>MAAPVVAPPGVVVSRANKRSGAGPGGSGGGGARGAEEEPPPPLQAVLVADSFDRRFFPISKDQPRVLLPLANVALIDYTLEFLTATGVQETFVFCCWKAAQIKEHLLKSKWCRPTSLNVVRIITSELYRSLGDVLRDVDAKALVRSDFLLVYGDVISNINITRALEEHRLRRKLEKNVSVMTMIFKESSPSHPTRCHEDNVVVAVDSTTNRVLHFQKTQGLRRFAFPLSLFQGSSDGVEVRYDLLDCHISICSPQVAQLFTDNFDYQTRDDFVRGLLVNEEILGNQIHMHVTAKEYGARVSNLHMYSAVCADVIRRWVYPLTPEANFTDSTTQSCTHSRHNIYRGPEVSLGHGSILEENVLLGSGTVIGSNCFITNSVIGPGCHIGDNVVLDQTYLWQGVRVAAGAQIHQSLLCDNAEVKERVTLKPRSVLTSQVVVGPNITLPEGSVISLHPPDAEEDEDDGEFSDDSGADQEKDKVKMKGYNPAEVGAAGKGYLWKAAGMNMEEEEELQQNLWGLKINMEEESESESEQSMDSEEPDSRGGSPQMDDIKVFQNEVLGTLQKGKEENISCDNLVLEINSLKYAYNISLKEVMQVLSHVVLEFPLQQMDSPLDSSRYCALLLPLLKAWSPVFRNYIKRAADHLEALAAIEDFFLEHEALGISMAKVLMAFYQLEILAGETILSWFSQRDTTDKGQQLRKNQQLQRFIQWLKEAEEESSEDD[2x];>MHHHHHHGGGSENLYFQSPGSAAKGSELSERIESFVETLKRGGGPRSSEEMARETLGLLRQIITDHRWSNAGELMELIRREGRRMTAAQPSETTVGNMVRRVLKIIREEYGRLHGRSDESDQQESLHKLLTSGGLNEDFSFHYAQLQSNIIEAINELLVELEGTMENIAAQALEHIHSNEVIMTIGFSRTVEAFLKEAARKRKFHVIVAECAPFCQGHEMAVNLSKAGIETTVMTDAAIFAVMSRVNKVIIGTKTILANGALRAVTGTHTLALAAKHHSTPLIVCAPMFKLSPQFPNEEDSFHKFVAPEEVLPFTEGDILEKVSVHCPVFDYVPPELITLFISNIGGNAPSYIYRLMSELYHPDDHVL[2x];>[2x]MAAVAVAVREDSGSGMKAELPPGPGAVGREMTKEEKLQLRKEKKQQKKKRKEEKGAEPETGSAVSAAQCQVGPTRELPESGIQLGTPREKVPAGRSKAELRAERRAKQEAERALKQARKGEQGGPPPKASPSTAGETPSGVKRLPEYPQVDDLLLRRLVKKPERQQVPTRKDYGSKVSLFSHLPQYSRQNSLTQFMSIPSSVIHPAMVRLGLQYSQGLVSGSNARCIALLRALQQVIQDYTTPPNEELSRDLVNKLKPYMSFLTQCRPLSASMHNAIKFLNKEITSVGSSKREEEAKSELRAAIDRYVQEKIVLAAQAISRFAYQKISNGDVILVYGCSSLVSRILQEAWTEGRRFRVVVVDSRPWLEGRHTLRSLVHAGVPASYLLIPAASYVLPEVSKVLLGAHALLANGSVMSRVGTAQLALVARAHNVPVLVCCETYK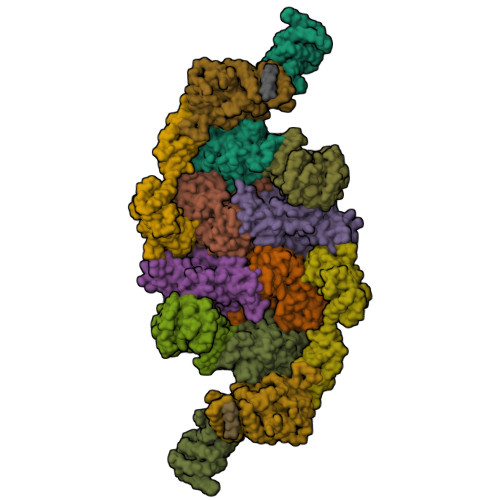FCERVQTDAFVSNELDDPDDLQCKRGEHVALANWQNHASLRLLNLVYDVTPPELVDLVITELGMIPCSSVPVVLRVKSSDQ;>MDDKELIEYFKSQMKEDPDMASAVAAIRTLLEFLKRDKGETIQGLRANLTSAIETLCGVDSSVAVSSGGELFLRFISLASLEYSDYSKCKKIMIERGELFLRRISLSRNKIADLCHTFIKDGATILTHAYSRVVLRVLEAAVAAKKRFSVYVTESQPDLSGKKMAKALCHLNVPVTVVLDAAVGYIMEKADLVIVGAEGVVENGGIINKIGTNQMAVCAKAQNKPFYVVAESFKFVRLFPLNQQDVPDKFKYKADTLKVAQTGQDLKEEHPWVDYTAPSLITLLFTDLGVLTPSAVSDELIKLYL[2x];>MEFQAVVMAVGGGSRMTDLTSSIPKPLLPVGNKPLIWYPLNLLERVGFEEVIVVTTRDVQKALCAEFKMKMKPDIVCIPDDADMGTADSLRYIYPKLKTDVLVLSCDLITDVALHEVVDLFRAYDASLAMLMRKGQDSIEPVPGQKGKKKAVEQRDFIGVDSTGKRLLFMANEADLDEELVIKGSILQKHPRIRFHTGLVDAHLYCLKKYIVDFLMENGSITSIRSELIPYLVRKQFSSASSQQGQEEKEEDLKKKELKSLDIYSFIKEANTLNLAPYDACWNACRGDRWEDLSRSQVRCYVHIMKEGLCSRVSTLGLYMEANRQVPKLLSALCPEEPPVHSSAQIVSKHLVGVDSLIGPETQIGEKSSIKRSVIGSSCLIKDRVTITNCLLMNSVTVEEGSNIQGSVICNNAVIEKGADIKDCLIGSGQRIEAKAKRVNEVIVGNDQLMEI[2x];>MPGLSCRFYQHKFPEVEDVVMVNVRSIAEMGAYVSLLEYNNIEGMILLSELSRRRIRSINKLIRIGRNECVVVIRVDKEKGYIDLSKRRVSPEEAIKCEDKFTKSKTVYSILRHVAEVLEYTKDEQLESLFQRTAWVFDDKYKRPGYGAYDAFKHAVSDPSILDSLDLNEDEREVLINNINRRLTPQAVKIRADIEVACYGYEGIDAVKEALRAGLNCSTENMPIKINLIAPPRYVMTTTTLERTEGLSVLSQAMAVIKEKIEEKRGVFNVQMEPKVVTDTDETELARQMERLERENAEVDGDDDAEEMEAKAED[2x];>MAGGEAGVTLGQPHLSRQDLTTLDVTKLTPLSHEVISRQATINIGTIGHVAHGKSTVVKAISGVHTVRFKNELERNITIKLGYANAKIYKLDDPSCPRPECYRSCGSSTPDEFPTDIPGTKGNFKLVRHVSFVDCPGHDILMATMLNGAAVMDAALLLIAGNESCPQPQTSEHLAAIEIMKLKHILILQNKIDLVKESQAKEQYEQILAFVQGTVAEGAPIIPISAQLKYNIEVVCEYIVKKIPVPPRDFTSEPRLIVIRSFDVNKPGCEVDDLKGGVAGGSILKGVLKVGQEIEVRPGIVSKASEGKLMCKPKFSKIVSLFAEHNDLQYAAPGGLIGVGTKIDPTLCRADRMVGQVLGAVGALPEIFTELEISYFLLRRLLGVRTEGDKKAAKVQKLSKNEVLMVNIGSLSTGGRVSAVKADLGKIVLTNPVCTEVGEKIALSRRVEKHWRLIGWGQIRRGVTIKPTVDDD[2x]>LSVDTSEYNRPLIHFTPEKGWMNDPNGLFYDKTAKLWHLYFQYNPNATAWGQPLYWGHATSNDLVHWDEHEIAIGPEHDNEGIFSGSIVVDHNNTSGFFNSSIDPNQRIVAIYTNNIPDNQTQDIAFSLDGGYTFTKYENNPVIDVSSNQFRDPKVFWHEDSNQWIMVVSKSQEYKIQIFGSANLKNWVLNSNFSSGYYGNQYECPGLIEVPIENSDKSKWVMFLAINPGSPLGGSINQYFVGDFDGFQFVPDDSQTRFVDIGKDFYAFQTFSEVEHGVLGLAWASNWQYADQVPTNPWRSSTSLARNYTLRYVHTNAETKQLTLIQNPVLPDSINVVDKLKKKNVKLTNKKPIKTNFKGSTGLFDFNITFKVLNLNVSPGKTHFDILINSQELNSSVDSIKIGFDSSQ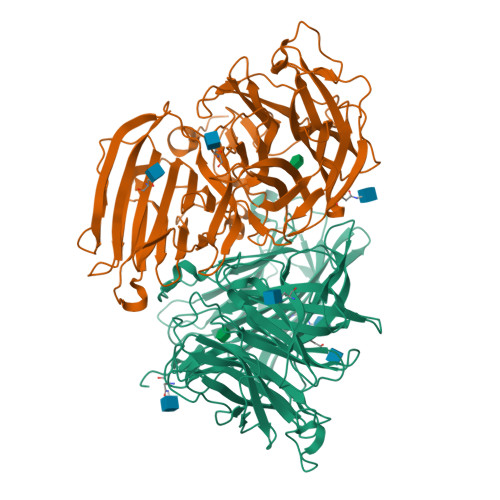SSFYIDRHIPNVEFPRKQFFTDKLAAYLEPLDYDQDLRVFSLYGIVDKNIIELYFNDGTVAMTNTFFMGEGKYPHDIQIVTDTEEPLFELESVIIRELNK[2x]> AEGSSSIYDNEGNFLFKVEGKFPPQPKKSSDYSWIEKVLEMGLQ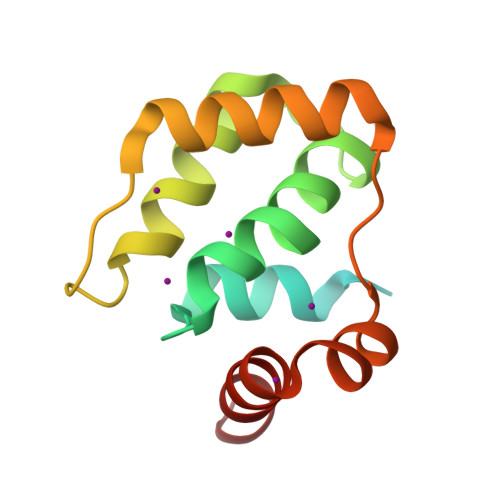DSRKRFILYVASRYLVNVKGVNEDEALQTLKEFYYKLQSGKVYESWLKSVINGVKKKGLLPWSLKRIEERDKEMYNEIIRVLKNS2-{4-[3-(5H-dibenzo[b,f]azepin-5-yl)propyl]piperazin-1-yl}ethyl beta-D-glucopyranoside | C29 H39 N3 O6 | 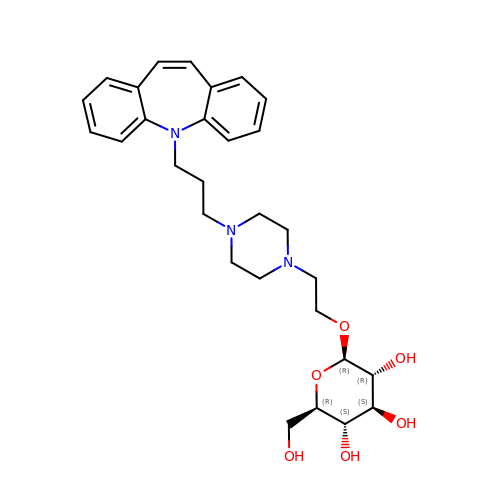GVUGRCGKZRTSLY-XYPQWYOHSA-N> MNHKVHHHHHHIEGRHMDGILDHGLHARFLRGLSAAPDGAAVRIGTTSVSYRHLHRTALLWAGALTAAGARSVGVLAGKSATGYAGILAALYAGAAVVPLRPDFPAARTREVLRASDADVLIADRAGLPVLAGALAGDGAADVPVLAPDALDGELPEGVARLVPRPELSLSEPARCKPADPAYLLFTSGSTGRPKGVVITHGATGHYFDVMERRYDFGASDVFSQAFDLNFDCAVFDLFCAWGAGATVVPVPPPAYRDLPGFITAQGITVWFSTPSVIDLTRRLGALDGPRMPGLRWSLFAGEALKCRDAADWRAAAPGATLENLYGPTELTITVAAHRWDDEESPRAAVNGLAPIGAVNDGHDHLLLGPDGDPSPDEGELWVTGPQLAAGYLDPADERGRFAERDGRRWYRTGDRVRRAPGGDLVYVGRLDSQLQVHG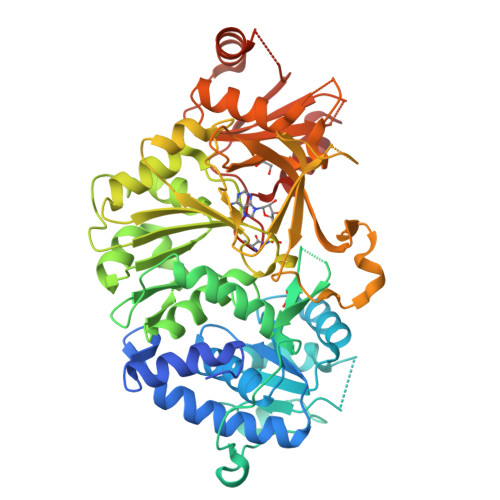WRVEPAEVEHAVRACGADDAVVVGVDTPGGTELVAFYTGIPVEPRELVRRLREVVPDGVLPRHFRHLDAFPLNANRKTDRLRLTTMAADGYGPRSGPAL>[2x]GMNASLEVPTATSVRAIPAKLMIDNRVVINNHLKRTRGGKISFTHLLGYAIVQAVKKFPNMNRHFAVVDGKPTAITPAHTNLGLAIDLQGKDGNRSLVVAAIKRCETMRFGQFIAAYEDIVRRARDGKLTAEDFSGVTISLTNPGTLGTVHSVPRLMQGQGAIIGAGAMEYPAEFQGASEERIADLGIGKLITLTSTYDHRIIQGAESGDFLRTIHQLLLDDDFFDEIFRELGIPYEPVRWRTDNPDSIEDKNARVIELIAAYRNRGHLMADIDPLRLDNTRFRSHPDLDVNSHGLTLWDLDREFKVDGFAGVQRKKLRDILSVLRDAYCRHVGVEYTHILEPEQQRWIQERVETKHDKPTVAEQKYILSKLNAAEAFETFLQTKYVGQKRFSLEGAETVIPMMDAVIDQCAEHGLDEVVIAMPHRGRLNVLANIVGKPYSQIFSEFEGNLNPSQAHGSGDVKYHLGATGTYIQMFGDNDIEVSLTANPSHLEAVDPVLEGLVRAKQDLLDTGEEGSDNRFSVVPLMLHGDAAFAGQGVVAETLNLALLRGYRTGGTIHIVVNNQIGFTTAPTDSRSSEYCTDVAKMIGAPIFHVNGDDPEACAWVARLAVDFRQAFKKDVVIDMLCYRRRGHNEGDDPSMTQPYMYDVIDTKRGSRKAYTEALIGRGDISMKEAEDALRDYQGQLERVFNEVRELEKHEIEPSESVEADQQIPSKLATAVDKAMLQRIGDAHLALPEGFTVHPRVRPVLEKRREMAYEGRIDWAFAELLALGSLIAEGKLVRLSGQDTQRGTFTQRHAVIVDRKTGEEFTPLQLLATNPDGTPTGGKFLVYNSALSEFAAVGFEYGYSVGNPDAMVLWEAQFGDFVNGAQSIIDEFISS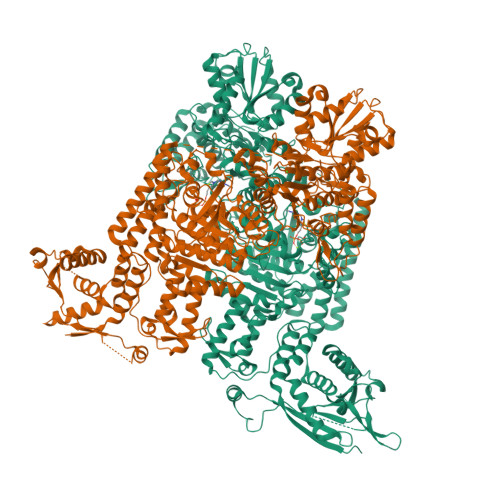GEAKWGQLSDVVLLLPHGHEGQGPDHTSGRIERFLQLWAEGSMTIAMPSTPANYFHLLRRHGKDGIQRPLIVFTPKSMLRNKAAVSDIRDFTESKFRSVLEEPMYTDGEGDRNKVTRLLLTSGKIYYELAARKAKENREDVAIVRIEQLAPLPRRRLAETLDRYPNVKEKFWVQEEPANQGAWPSFGLTLPEILPDHFTGLKRISRRAMSAPSSGSSKVHAVEQQEILDTAFG> MKYRGPEDKLIVFTFYKESKKKRHFFPFFLQKISYLFQNIYLYFLTTFVQSILIDQAG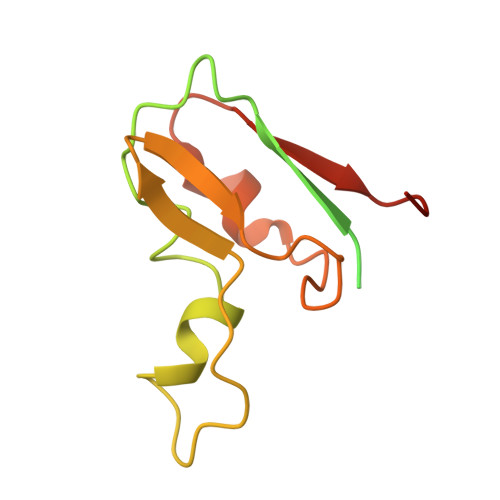ATNMAFAVHVNMERCTGCNNCVVACPVNALELNTVNPSSTDKIYKVINGDAVILDVKHELCAGCGICVDACPYDVIQLSGQPPQAVEA>MTTRDAATIKALLSHAHEAQRSGDVLASERACWRVLQIAPDNSEALHLLGLLHGECGNYGLAATLLRRAVALDPGEASYHYNLGNVLVASGQVERGITSLHHALELRPDYHRAHSGLYVALHYSALYDPRA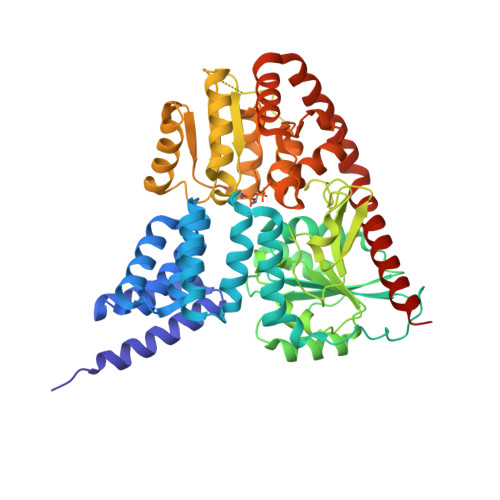RHILALDWARRYADPLTPVPATPVDPDPHRRLRIGYVSGELRCHPVGYFLEPVIEAHDRTAYEVYCYSNDPRSDALTDRLRALSDRWRDVWPLTDAELCELVRRDGIDILVDLSWHLGMHRLFAFARRPAPVQVTWLAAINTTGMRAMDYLVGDQHLCPPGSDELYTERLVRLSRFYLPCNPPPDLPGWAPADPLGRGFPVFGCFNRLSMIGPEVLDLWAKILLALPRARLRLIATGLQDPVTSSRLMRALEGRGVAGERLELLSPMPRTDLLATYNDIDVALDTLPYSGCTTSLEALWMGVPVVTLEGADMAGRATSSLLRWAGLQELVSRTQEEYIDIALGLGRDLGTLARLREHLRRWLRSVSMSDQGSFTAELEDAYRRMWRDACQTAAGRQGA[4x]>[2x]GSHMGDFVVVYTDGCCSSNGRRRPRAGIGVYWGPGHPLNVGIRLPGRQTNQRAEIHAACKAIEQAKTQN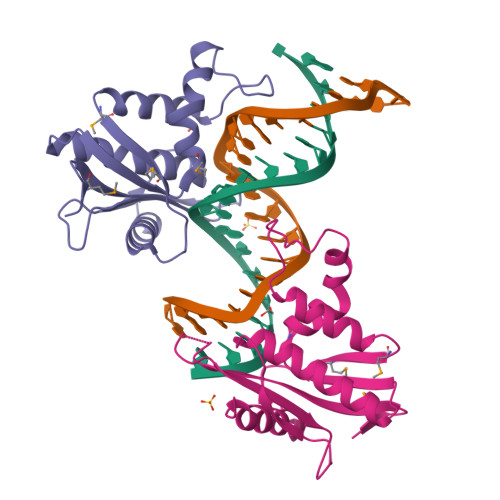INKLVLYTNSMFTINGITNWVQGWKKNGWKTSAGKEVINKEDFVALERLTQGMDIQWMHVPGHSGFIGNEEADRLAREGAKQSED>TPMRSPIIWINGPFGVGKTHTAHTLHERLPGSFVFEPEE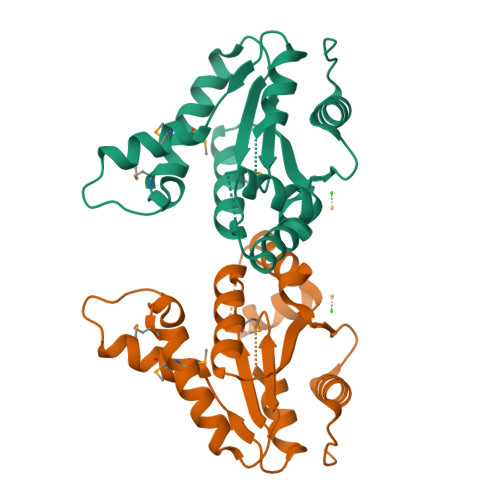MGQALRKLTPGFSGDPQEHPMWIPLMLDALQYASREAAGPLIVPVSISDTARHRRLMSGLKDRGLSVHHFTLIAPLNVVLERLRRDGQPQVNVGTVEDRLNELRGEQFQTHIDTAGLGTQQVAEQIAAQVGLTLAPPPQGALHW[2x]>[2x]QSTVPAWGQCGGSVPASSAGKLQFAGVNIAGFDFGCGSDGTCNASGAWPPLTQYYGADGAGQMKHFVDDDGFNVFRLPVGWQFITDGVAGGDIDEDNWAEYDALVQACLDAGASCIVDVHNYARFNGEIIGQGGPTNQDFAALWSSIAAKYADNDKIIFGVMNEPHDVPDINLWADSVQAAVTAIRQAGATSQIILLPGNNWTSAETFVSNGSADAL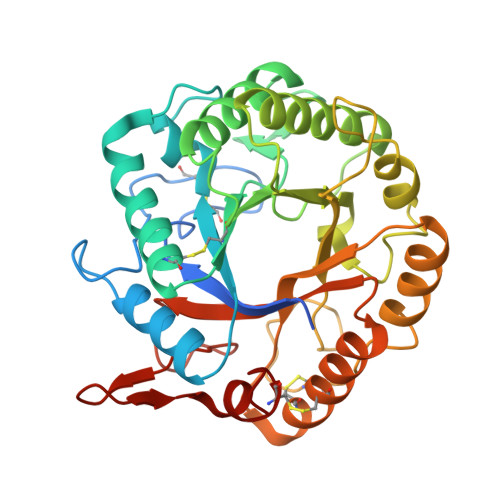KKVTNPDGSVTNLIFDVHKYLDSDNSGTHEECTTNNIDNAWAPLAEWLRCNGRQAFNTETGGGNVASCETFMCQQVAYQNANSDVFLGYVGWAAGNFYQGYVLGEVPTDTNGVWTDTALVSACLAPNAQK> NDHINLKVAGQDGSVVQFKIKRHTPLSKLMKAYCERQGLSMRQIRFRFDG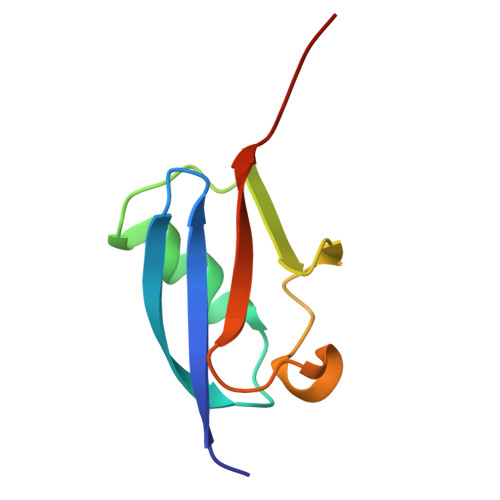QPINETDTPAQLEMEDEDTIDVFQQQTGGVY> GASNSYAIPE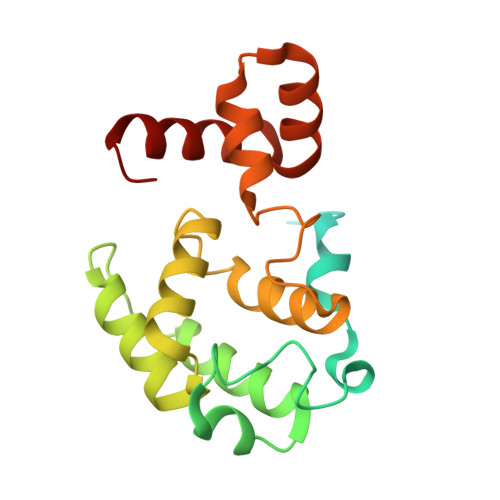NELLDEDTMNFISSLKNDLSNISNSLPFEYPHEIAEAIRSDFSNEDIYDNIDPDTISFPPKIATTDLFLPLFFHFGSTRQFMDKLHEVISGDYEPSQAEKLVQDLCDETGIRKNFSTSILTCLSGDLMVFPRYFLNMFKDNVNPPPNVPGIWTHDDDESLKSNDQEQIRKLVKKHGTGRMEMRKRFFEKDLL> RAVDLVDDSNDVDNSIEAEEEKPRNRAFEADWLKFTKTPPTKLQQADGATIEIVCEMMGSQVPSIQWVVGHLPRSELDDLDSNQVAEEAPSAIVRVRSSHIIDHVLSEARTYTCVGRTGSKTIYASTVVHPPRSSRLTPEKTYPGAQKPRIIYTEKTHLDLMGSNIQLPCRVHARPRAEITWLNNENKEIVQGHRHRVLANGDLLISEIKWEDMGNYKCIARNVVGKDTADTFVYPVLNEED;> GPETLCGAELVDALQ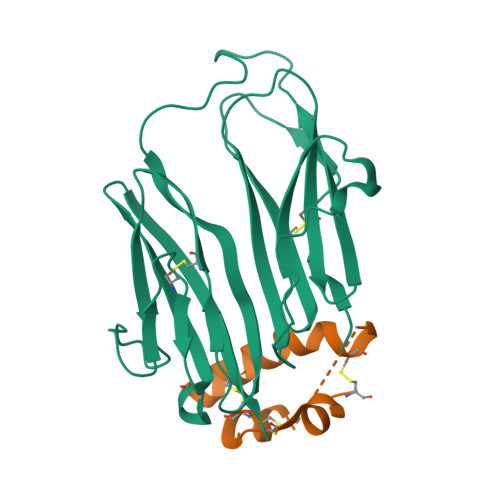FVCGDRGFYFNKPTGYGSSSRRAPQTGIVDECCFRSCDLRRLEMYCAPLKPAKSA> SEISRQEFQRRRQALVEQMQPGSAALIFAAPEVTRSADSEYPYR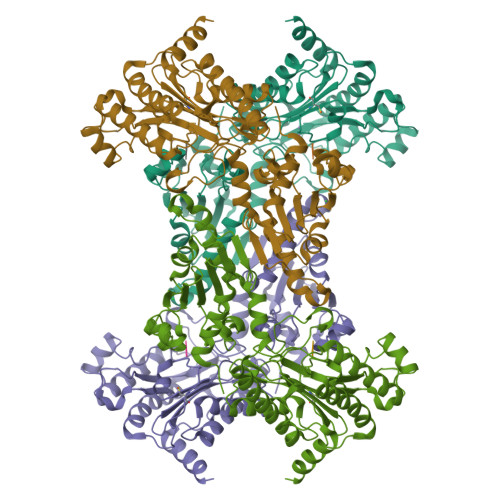QNSDFWYFTGFNEPEAVLVLIKSDDTHNHSVLFNRVRDLTAEIWFGRRLGQDAAPEKLGVDRALAFSEINQQLYQLLNGLDVVYHAQGEYAYADVIVNSALEKLRKGSRQNLTAPATMIDWRPVVHEMRLFKSPEEIAVLRRAGEITAMAHTRAMEKCRPGMFEYHLEGEIHHEFNRHGARYPSYNTIVGSGENGCILHYTENECEMRDGDLVLIDAGCEYKGYAGDITRTFPVNGKFTQAQREIYDIVLESLETSLRLYRPGTSILEVTGEVVRIMVSGLVKLGILKGDVDELIAQNAHRPFFMHGLSHWLGLDVADVGVYGQDRSRILEPGMVLTVEPGLYIAPDAEVPEQYRGIGIRIEDDIVITETGNENLTASVVKKPEEIEALMVAARKQ;> VPL>AQYEDGKQYTTLEKPVAGAPQVLEFFSFFCPYCYQFEEVLHISDNVKKKLPEGVKMTKYHVNFMGGD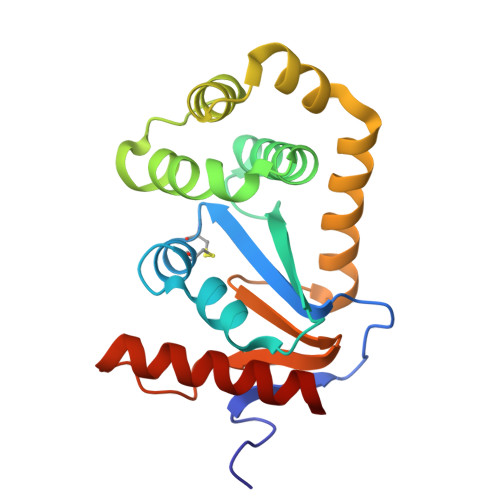LGKDLTQAWAVAMALGVEDKVTVPLFEGVQKTQTIRSASDIRDVFINAGIKGEEYDAAWNSFVVKSLVAQQEKAAADVQLRGVPAMFVNGKYQLNPQGMDTSNMDVFVQQYADTVKYLSEKK[2x]> GLGDELEEVIVEKTKQTVASISSGPKHTQKVPILTANETGATMPVLPSDSIETRTTYMHFNGSETDVECFLGRAACVHVTEIQNKDATGIDNHREAKLFNDWKINLSSLVQLRKKLELFTYVRFDSEYTILATASQPDSANYSSNLVVQAMYVPPGAPNPKEWDDYTWQSASNPSVFFKVGDTSRFSVPYVGLASAYNYFYDGYSHDDAETQYGITVLNHMGSMAFRIVNEHDEHKTLVKIRVYHRAKHVEAWIPRAPRALPYTSIGRTNYPKNTEPVIKKRKGDIKSY;> SPNVEACGYSDRVQQITLGNSTITTQEAANAVVCYAEWPEYLPDVDASDVNKTSKPDTSVCRFYTLD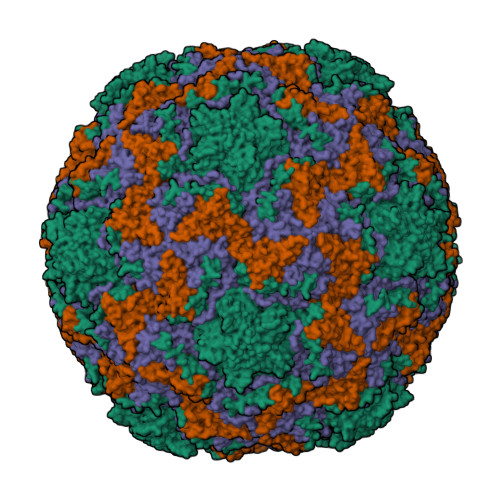SKTWTTGSKGWCWKLPDALKDMGVFGQNMFFHSLGRSGYTVHVQCNATKFHSGCLLVVVIPEHQLASHEGGNVSVKYTFTHPGERGIDLSSANEVGGPVKDVLYNMNGTLLGNLLIFPHQFINLRTNNTATIVIPYINSVPIDSMTRHNNVSLMVIPIAPLTVPTGATPSLPITVTIAPMCTEFSGIRSKSIVPQ;> GLPTTTLPGSGQFLTTDDRQSPSALPNYEPTPRIHIPGKVHNLLEIIQVDTLIPMNNTHTKDEVNSYLIPLNANRQNEQVFGTNLFIGDGVFKTTLLGEIVQYYTHWSGSLRFSLMYTGPALSSAKLILAYTPPGARGPQDRREAMLGTHVVWDIGLQSTIVMTIPWTSGVQFRYTDPDTYTSAGFLSCWYQTSLILPPETTGQVYLLSFISACPDFKLRLMKDTQTISQTVALTE;> GAQVSTQKSGSHENQNILTNGSNQTFTVINYYKDAASTSSAGQSLSMDPSKFTEPVKDLMLKGAPALN> MLFEGDKFVGSFENAAAGTFVLDMYAYERLANS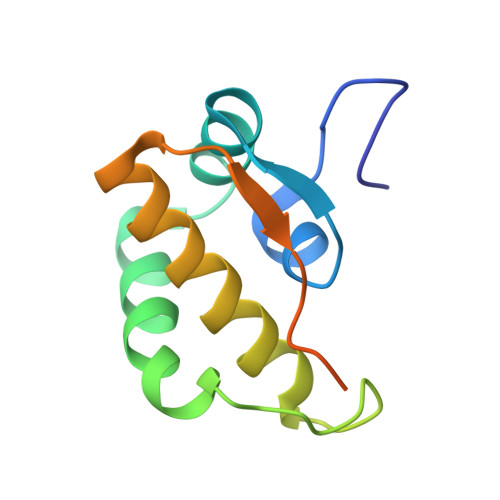ISTEKLRQYASTYNKYKYYSGSASEADYRLACFAHLAKAMMDYASNHNDTLYTPPTVSYNSTLQLEHHHHHHHH>GCGCCGGUUAGGCAGAGGUGGGUGGUGUGGAGGAGUAUCUGUCCGGCGC[2x]

Beetroot is a homodimeric in vitro selected RNA that binds and activates DFAME, a conditional fluorophore derived from GFP. It is 70% sequence-identical to the previously characterized homodimeric aptamer Corn, which binds one molecule of its cognate fluorophore DFHO at its interprotomer interface. Each protomer comprises two duplex segments (P1 and P2) separated by an irregular junction (J1/2) and a mixed connectivity quadruplex. The latter has three canonical G-quartet tiers (T1, T2, and T3) and one mixed-composition (G•U•A•A) tier (T4).

We have now determined the Beetroot-DFAME co-crystal structure at 1.95 Å resolution, discovering that this RNA homodimer binds two molecules of the fluorophore, at sites separated by ~30 Å. The structural elements of the dimer form a 100 Å-tall continuous coaxial stack, with T1 and t1 of the two RNAs stacking on each other to form the interprotomer interface. Each fluorophore stacks between the face of the G-quartet distal from the dimer interface, and the adjacent duplex P2. DFAME binds the RNA with its two rings and its methylacrylate substituent coplanar, sandwiched between the G17•U26•A34•A37 (T4) tetrad and the terminal A16•U38 Watson-Crick pair of P2. The phenyl ring of DFAME stacks between G17 and A16, while its methylacrylate portion between U26 and A37 of T4 of U38 of P2. Remarkably, the fluorophore makes no hydrogen bonds to the RNA. The binding site is comparatively open, and the RNA only buries 40% of the total 523 Å2 solvent-accessible surface area of DFAME. Co-axial stacking of the two Beetroot protomers results in an eight-tiered quadruplex spanning the dimer interface. Five octacoordinated K+ ions lie on its four-fold symmetry axis, equidistant from the planes of successive canonical G-quartets. Fluorophore binding is exothermic, with an RNA protomer:fluorophore molar ratio of 1:1.> GSHMTVQLNHTIVAAHDKKASARFLADILGLEVSPQYGPFIPVEI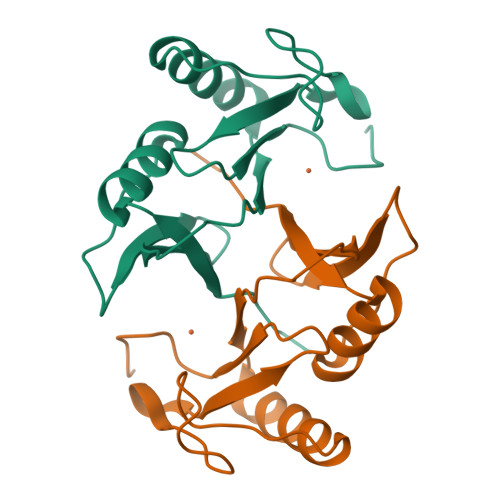PNGVSLDYLDSRGAITPQHYAFLVSEDDFDTIFGRIREAGLTYWADPYHRRPGEINHNDGGRGAYFEDPNGHNLEILTRPYGSGG>GHMNALPNRQPAGTTSSLVVRNLKKRYGSRTVVKDVSLDVKSGEVVGLLGPNGAGKTTSFYMIVGLVPLDAGDISLNGSPISLMPIHKRASLGLSYLPQEASVFRKLTVEQNVRAVLELQHDENGKRLSK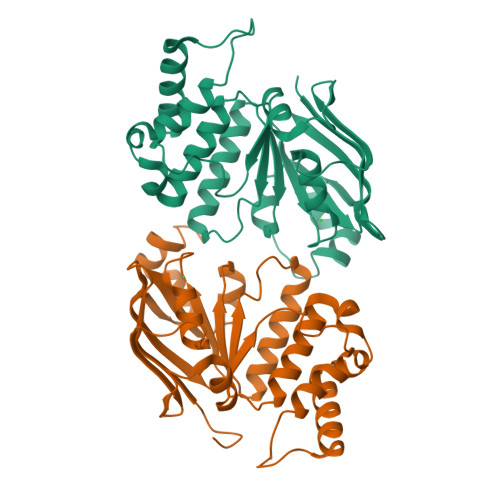DAIGARTEALLEELQIAHLRENPALSLSGGERRRVEIARALASNPSFILLDEPFAGVDPIAVLEIQKIVKFLKQRNIGVLITDHNVRETLGICDHAYIISDGSVLASGAPKEIIENESVRRVYLGEHFRM[2x]> GHHHHHHHHHHSSGHIEGRHMPAAPSPAPAGAVAGGPAAGVPAAASGAAEAAMPLPAALPGALAGSHAPRLPLAAGGRLARTRAVREFFDYCLTAQGELTPAALDALVRREIAAQLDGSPAQAEALGVWRRYRAYFDALAQLPGDGAVLGDKLDPAAMQLALDQRAALADRTLGEWAEPFFG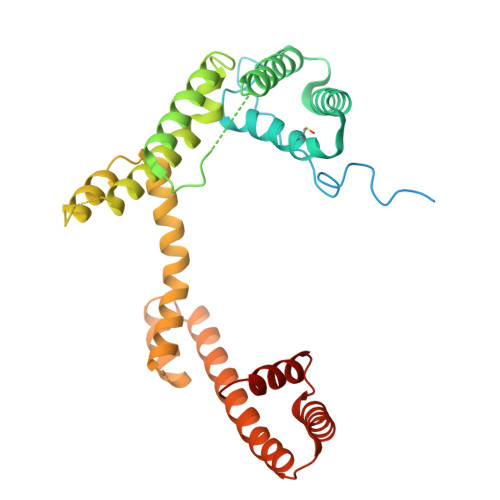DEQRRQRHDLERIRIANDTTLSPEQKAARLAALDAQLTPDERAQQAALHAQQDAVTKIADLQKAGATPDQMRAQIAQTLGPEAAARAAQMQQDDEAWQTRYQAYAAERDRIAAQGLAPQDRDARIAQLRQQTFTAPGEAIRAASLDRGAG> SLPENAPNAVSNPQQFITPATALSAEEYNVHEALGETEELELDEFPVLVFKGNVPVDSVTSIPLDLATIYDFAWDGEQNAISQKFQRFAHLIPKSAGGFGPVIGNYTITANLPTGVAGRILHNCLPGDCVDLAVSRIFGLKSLLGVAGTAVSAIGGPLLNGLVNTAAPILSGAAHAIGGNVVGGLADAVIDIGSNLLTPKEKEQPSANSSAISGDIPISRFVEMLKYVKENYQDNPVFPTLLVEPQNFISNAMTALKTIPIEVFANMRNVKVERNLFDRTVVPTVKEATLADIVIPNHMYGYILRDFLQNKRAFQSGTKQNVYFQQFLTVLSQRNIRTHITLNDITSCSIDSESIANKIERVKHYLSTNSSGETTEEFSRTDTGLLPITTRKIVLGESKRRTERYVAE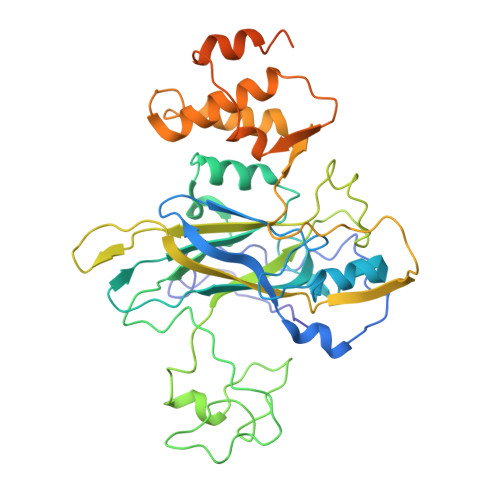TVFPSVRQ>MKGQETRGFQSEVKQLLHLMIHSLYSNKEIFLRELISNASDAADKLRFRALSNPDLYEGDGELRVRVSFDKDKRTLTISDNGVGMTRDEV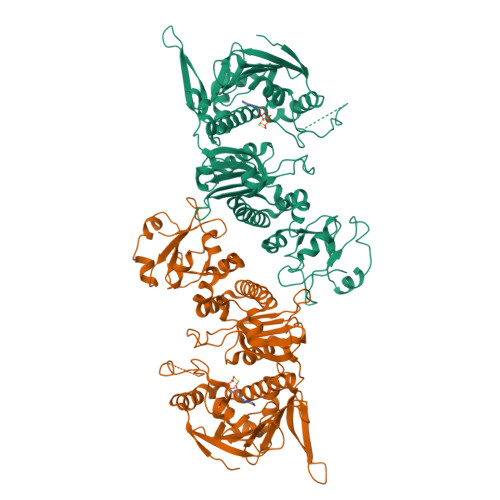IDHLGTIAKSGTKSFLESLGSDQAKDSQLIGQFGVGFYSAFIVADKVTVRTRAAGEKPENGVFWESAGEGEYTVADITKEDRGTEITLHLREGEDEFLDDWRVRSIISKYSDHIALPVEIEKREEKDGETVISWEKINKAQALWTRNKSEITDEEYKEFYKHIAHDFNDPLTWSHNRVEGKQEYTSLLYIPSQAPWDMWNRDHKHGLKLYVQRVFIMDDAEQFMPNYLRFVRGLIDSSDLPLNVSREILQDSTVTRNLRNALTKRVLQMLEKLAKDDAEKYQTFWQQFGLVLKEGPAEDFANQEAIAKLLRFASTHTDSSAQTVSLEDYVSRMKEGQEKIYYITADSYAAAKSSPHLELLRKKGIEVLLLSDRIDEWMMNYLTEFDGKPFQSVSKVDESLEKLADEVDESAKEAEKALTPFIDRVKALLGERVKDVRLTHRLTDTPAIVSTDADEMSTQMAKLFAAAGQ[2x]>[2x]LRDLVCYCRTRGCKRRERMNGTCRKGHLMHTLCCR

Mouse α-defensins, better known as cryptdins, are host protective antimicrobial peptides produced in the intestinal crypt by Paneth cells. Mammalian defensins of 2 to 5 kDa in size are rich in Arg and/or Lys residues with three intramolecular disulfide bonds and are classified into α, β, and θ subfamilies according to their disulfide topology and sites of expression. Cryptdins are initially synthesized as inactive precursors, i.e., procryptdins, which are proteolytically processed to their active mature forms by matrix metalloproteinase 7 (MMP-7 or matrilysin). Based on sequence variability, the 17 cryptdins identified from a single jejunal crypt can be grouped into three subclasses: Crp1-like, Crp4, and Crp5, of which Crp1-like peptides are highly similar and form the largest group of cryptdins comprising Crp1 to Crp3 and Crp6 to Crp17 (29, 37).

However, only the structure of Crp14 has been determined by X-ray crystallography to a high resolution of 1.67 Å. Crp14 adopts a disulfide-stabilized, three-stranded β-sheet core structure and forms a noncanonical dimer stabilized by asymmetrical interactions between the two β1 strands in parallel. Arg9 and Glu17 form a salt bridge that is conserved in all mammalian α-defensins. This salt bridge rigidifies the first loop connecting β1-β2 (56, 66) and is additionally stabilized by a Lys14 O accepting H-bond from Glu17 N and a Lys14 N donating H-bond to Glu17 Oε1. As shown in the electrostatic potential map, Crp14 is clearly amphiphilic with a cluster of positively charged residues well segregated from a large hydrophobic surface. Crp14 crystallized in space group P6522 with two Crp14 molecules in the asymmetric unit that form an apparent dimer that is different from the dimers of other α-defensins with known crystal structures. Crp14 dimerization is mediated primarily by interactions between the two β1 strands in parallel, in contrast to the dimers of other known α-defensins that dimerize via the interactions of the two β2 strands in antiparallel. Four asymmetric main chain-main chain H-bonds form the basis of the dimer interface, i.e., Leu4a O-Leu4b N, Cys6a N-Leu4b O, Cys6a O-Cys6b N, and Cys8a N-Cys6b O. In addition, Asp3b N donates an H-bond to Asp3a Oδ1 and the side chain of Tyr7 packs against neighboring disulfide bonds in both copies. However, the total buried surface area (BSA) for both dimers is similar, 724 Å2 for the Crp14 dimer compared to 744 Å2 for HNP1. As shown in the dimeric structure of Crp14, the two side chains of Thr10 directly point toward each other, 8.3 Å apart between Thr10 Oγ1 atoms, such that a T10K variation may be energetically unfavorable for cryptdin dimerization due to electrostatic repulsion.>[4x]SGEYTEIALPFSYDGAGE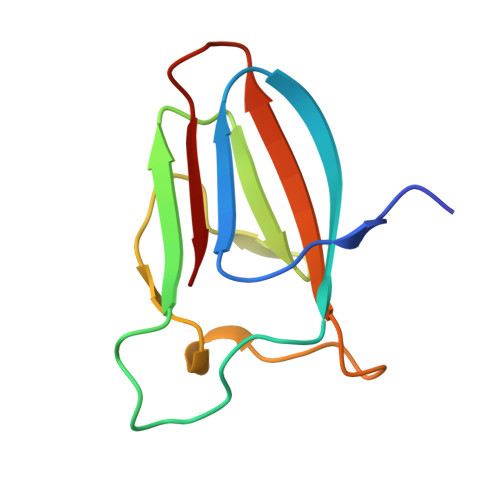YYWKTDQFSTDPNDWSRYVNSWNLDLLEINATDYTNVWVAQHQIPAASDGYWYIHYKSGVSWGHVEIK> SATTGARSASVGWAESLIGLHLGKVALITGGSAGIGGQIGRLLALSGARVMLAARDRHKLEQMQAMIQSELAEVGYTDVEDRVHIAPGCDVSSEAQLADLVERTLSAFGTVDYLINNAGIAGVEEMVIDMPVEGWRHTLFANLISNYSLMRKLAPLMKKQGSGYILNVSSYFGGEKDAAIPYPNRADYAVSKAGQRAMAEVFARFLGPEIQINAIAPGPVEGDRLRGTGWRPGLFARRARLILENKRLNELHAALIAAARTDERSMHELVELLLPNDVAALEQNPAAPTALRELARRFRSEGDPAASSSSALLNRSIAAKLLARLHNGGYVLPADIFANLPNPPDPFFTRAQIDREARKVRDGIMGMLYLQRMPTEFDVAMATVYYLADRNVSG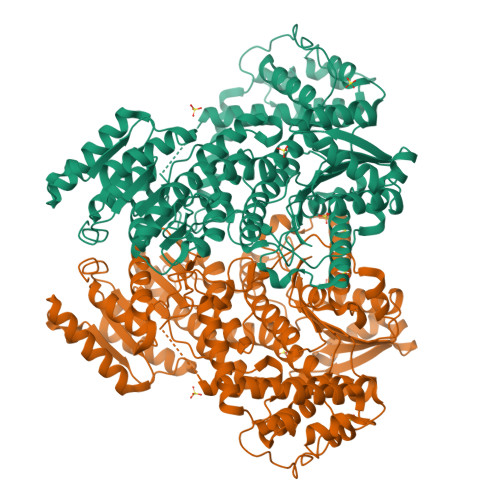ETFHPSGGLRYERTPTGGELFGLPSPERLAELVGSTVYLIGEHLTEHLNLLARAYLERYGARQVVMIVETETGAETMRRLLHDHVEAGRLMTIVAGDQIEAAIDQAITRYGRPGPVVCTPFRPLPTVPLVGRKDSDWSTVLSEAEFAELCEHQLTHHFRVARKIALSDGASLALVTPETTATSTTEQFALANFIKTTLHAFTATIGVESERTAQRILINQVDLTRRARAEEPRDPHERQQELERFIEAVLLVTAPLPPEADTRYAGRIHRGRAITV> GSSHSSANEDMPVERILEAELAVEPKTETYVEANMGLNPSSPNDPVTNICQAADKQLFTLVEWAKRIPHFSELPLDDQVILLRAGWNELLIASFSHRSIAVKDGILLATGLHVHRNSAHSAGVGAIFDRVLTELVSKMRDMQMDKTELGCLRAIVLFNPDSKGLSNPAEVEALREKVYASLEA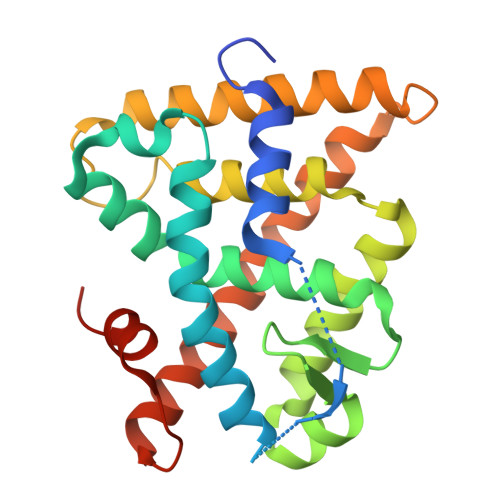YCKHKYPEQPGRFAKLLLRLPALRSIGLKCLEHLFFFKLIGDTPIDTFLMEMLEAPHQMT> EFETIERFMDCRIGRKGATGATTTIYAVEADGDPNAGFEKNKEPGEIQYLIKWKGWSHIHNTWETEETLKQQNVRGMKKLDNYKKKDQETKRWLKNASPEDVEYYNCQQELTDDLHKQYQIVERIIAHSNQKSAAGYP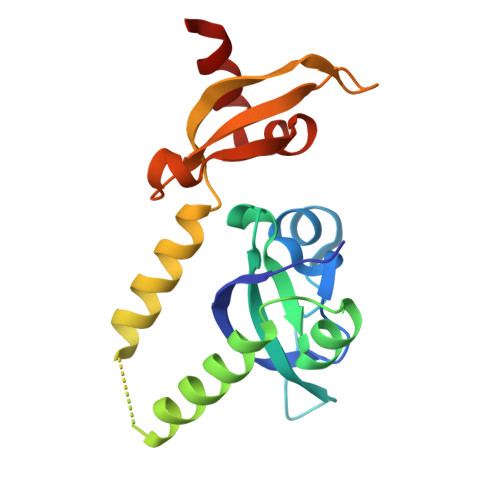DYYCKWQGLPYSECSWEDGALISKKFQACIDEYFSR methyl 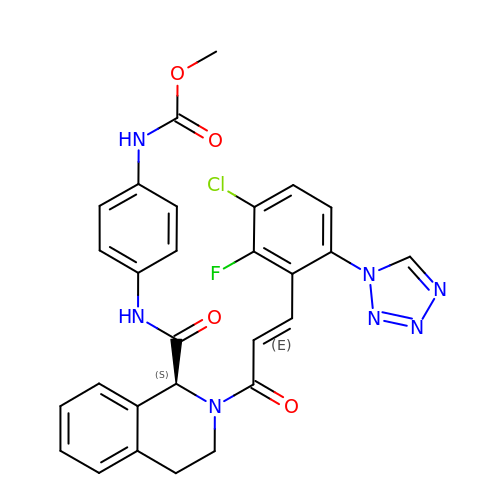~{N}-[4-[[(1~{S})-2-[(~{E})-3-[3-chloranyl-2-fluoranyl-6-(1,2,3,4-tetrazol-1-yl)phenyl]prop-2-enoyl]-3,4-dihydro-1~{H}-isoquinolin-1-yl]carbonylamino]phenyl]carbamate | C28 H23 Cl F N7 O4 | VNRXJEHYEMPJMV-ITMPFJHPSA-N>[2x]AKKKATETTDEDEDGGSEKKYRKCEKAGCTATCPVCFASASERCAKNGYTSRWYHLSCGEHFCNECFDHYYRSHKDGYDKYTTWKKIWT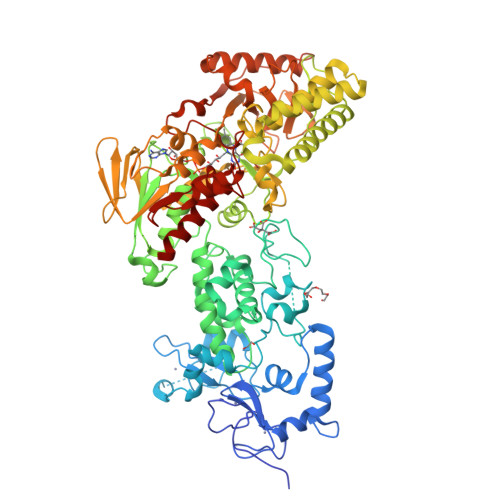SNGKTEPSPKAFMADQQLPYWVQCTKPECRKWRQLTKEIQLTPQIAKTYRCGMKPNTAIKPETSDHCSLPEDLRVLEVSNHWWYSMLILPPLLKDSVAAPLLSAYYPDCVGMSPSCTSTNRAAATGNASPGKLEHSKAALSVHVPGMNRYFQPFYQPNECGKALCVRPDVMELDELYEFPEYSRDPTMYLALRNLILALWYTNCKEALTPQKCIPHIIVRGLVRIRCVQEVERILYFMTRKGLINTGVLSVGADQYLLPKDYHNKSVIIIGAGPAGLAAARQLHNFGIKVTVLEAKDRIGGRVWDDKSFKGVTVGRGAQIVNGCINNPVALMCEQLGISMHKFGERCDLIQEGGRITDPTIDKRMDFHFNALLDVVSEWRKDKTQLQDVPLGEKIEEIYKAFIKESGIQFSELEGQVLQFHLSNLEYACGSNLHQVSARSWDHNEFFAQFAGDHTLLTPGYSVIIEKLAEGLDIQLKSPVQCIDYSGDEVQVTTTDGTGYSAQKVLVTVPLALLQKGAIQFNPPLSEKKMKAINSLGAGIIEKIALQFPYRFWDSKVQGADFFGHVPPSASKRGLFAVFYDMDPQKKHSVLMSVIAGEAVASVRTLDDKQVLQQCMATLRELFKEQEVPDPTKYFVTRWSTDPWIQMAYSFVKTGGSGEAYDIIAEDIQGTVFFAGEATNRHFPQTVTGAYLSGVREASKIAAF>MAHHHHHHHRSADQETEPGVPADLPAESDPAALERLAARYRRDGYVHVPGVLDAGEVAEYLAEARRLLAHEESVRWGSGAGTVMDYVADAQLGSDTMRRLATHPRIAALAEYLAGSPLRLFKLEVLLKENKEKDASVPTAPHHDAFAFPFSTAGTALTAWVALVDVPVERGCMTFVPGSHLLPDPDTGDEPWAGAFTRPGEIWMPRVTVPLR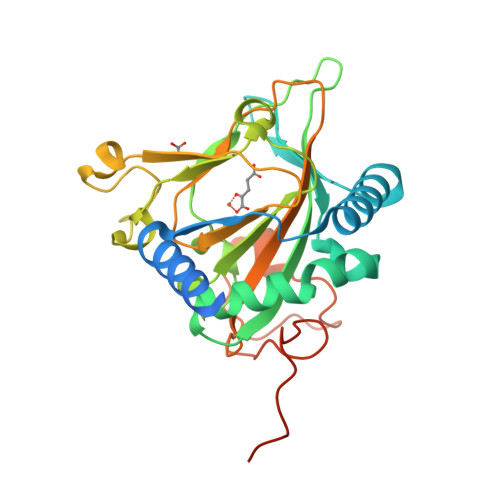AGDCTFHHARTVHSAGANSTDEPRLSTSAVYMDATAAYRPTGIAFLDDLPGTGADPLREGAPLTGDRFPLLRRPQTRQPAPARYPLPQQGHGS[4x]>MNAHSKEMAPLMGKRTTAPGGNPVVLTEKRPADLTPTKKSAHFFLEIEGFEPNPTVTKTSPPIFSKPMDSNIRQCLSGNCDDMDSPQSPQDDVTETPSNPNSPSANLAKEEQRQKKKRLKKRIFAAVSEGCVEELRELLQDLQDLCRRRRGLDVPDFLMHKLTASDTGKTCLMKALLNINPNTKEIVRILLAFAEENDILDRFINAEYTEEAYEGQTALNIAIERRQGDITAVLIAAGADVNAHAKGVFFNPKYQHEGFYFGETPLALAACTNQPEIVQLLMENEQTDITSQDSRGNNILHALVTVAEDFKTQNDFVKRMYDMILLRSGNWELETMRNNDGLTPLQLAAKMGKAEILKYILSREIKEKPLRSLSRKFTDWAYGPVSSSLYDLTNVDTTTDNSVLEIIVYNTNIDNRHEMLTLEPLHTLLHTKWKKFAKYMFFLSFCFYFFYNITLTLVSYYRPREDEDLPHPLALTHKMSWLQLLGRMFVLIWATCISVKEGIAIFLLRPSDLQSILSDAWFHFVFFVQAVLVILSVFLYLFAYKEYLACLVLAMALGWANMLYYTRGFQSMGMYSVMIQKVILHDVLKFLFVYILFLLGFGVALASLIEKCSKDKKDCSSYGSFSDAVLELFKLTIGLGDLNIQQNSTYPILFLFLLITYVILTFVLLLNMLIALMGETVENVSKESERIWRLQRARTILEFEKMLPEWLRSRFRMGELCKVADEDFRLCLRINEVKWTEWKTHVSFLNEDPGPIRRTADLNKIQDSSRSNSKTTLYAFDELDEFPETSVLVPRGS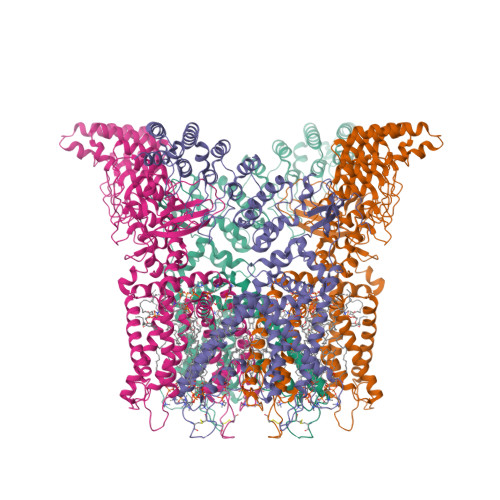AAAWSHPQFEK[4x]> GHMTPANIAGMVVFIDPGHNGANDASIGRQVPTGRGGTKNCQASGTSTNSGYPEHTFTWETGLRLRAALNALGVRTALSRGNDNALGPCVDERANMANALRPNAIVSLHADGGPASGRGFHVNYSAPPLNAIQAGPSVQFARIMRDQLQASGIPKANYIGQDGLYGRSDLAGLN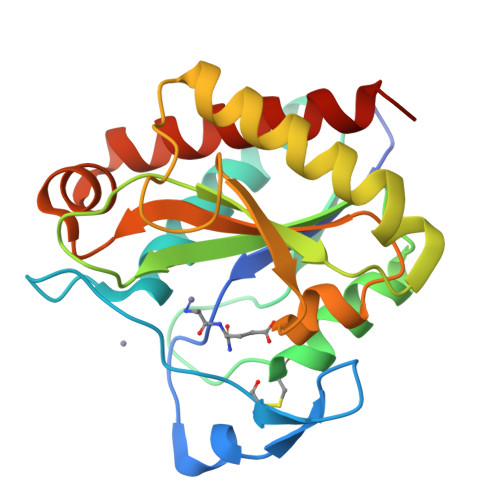LAQYPSILVELGNMKNPADSALMESAEGRQKYANALVRGVAGFLATQGQAR> MAIPKIASYQ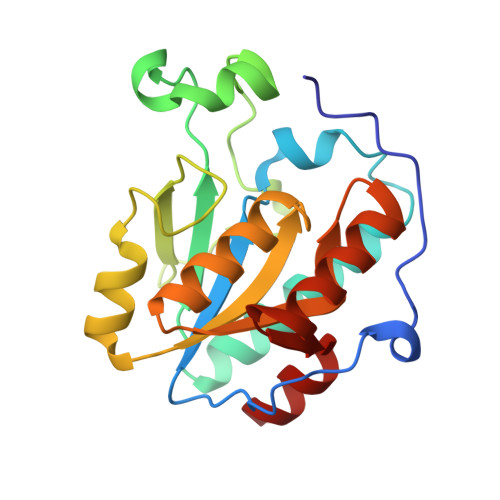VLPLESFPTNKVDWVIDPKKSVVLVHDLQAYFLNFFDKTLSPVPELLRNVNKVTESARSAGIPVVYTAQPANQDPNERALLTDFWGVGLTQDTEIVPEVSPQPEDIQYTKWRYSAFKKTPLLEWMKEEQRDQLVIVGVYGHIGILSTALDAFMLDIKPFVIGDAIADFSKEDHMNTLKYVASRSGSVKSVDEFISSVT>[3x]MVNTVNYFKQKLKTEQQIGMWVGLADGYCAEIAANVGYDWLLIDGEHAPNDVRSILAQLQSIAAYPSQAVVRPVSGDVPLIKQLLDIGAQTLLIPMVESAEQAELMVKATRYPPEGIRGVGAALARASRWNNISDYLQTADEQICLLVQVESKKGLDNLDEILNVDGVDGIFIGPADLSAALGY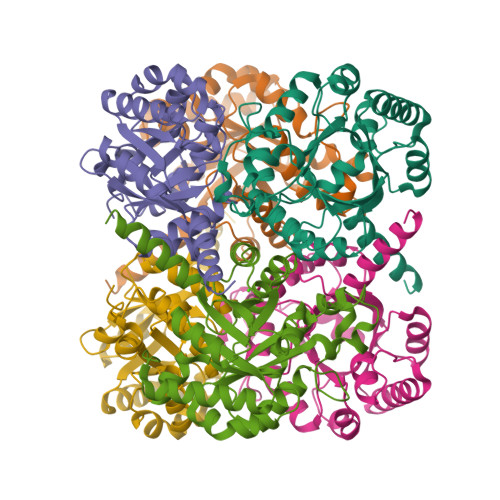RGNPGHEFVQNIIVQTIQKIRAAGKAAGILSADEKLAKQYLELGTEFVAVGVDTSLLMKSMKQLLSKFKNVDGPVSTSPSVY> AFDAFLKIDGIPGESSDDKHKDWIEIQSFAHKLEQPAQATASSAGGATAERVNHAAYEITHFLDKASPKIYEACCKGQHIKEITIELCRAGGDKVKYME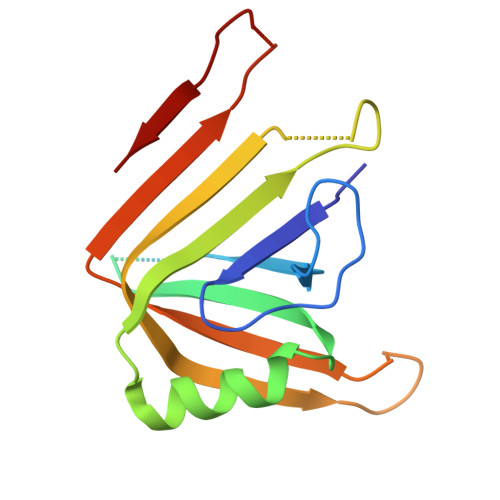IKMEQVLIAKVEPHGSANDNGFPSEKVSFTYGKIKWTYTQQKRADGAGGGNVSSG2-(pyridin-2-yl)-N-(5-{4-[6-({[3-(trifluoromethoxy)phenyl]acetyl}amino)pyridazin-3-yl]butyl}-1,3,4-thiadiazol-2-yl)acetamide 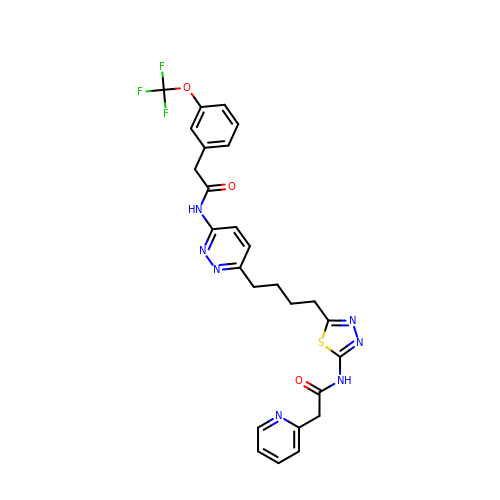| C26 H24 F3 N7 O3 S | PRAAPINBUWJLGA-UHFFFAOYSA-N> DSISLSLINEGPSYASKVSVGSNKQQQTVIIDTGSSDFWVVDSNAQCGKGVDCKSSGTFTPSSSSSYKNLGAAFTIRYGDGSTSQGTWGKDTVTINGVSITGQQIADVTQTSVDQGILGIGYTSNEAVYDTSGRQTTPNYDNVPVTLKKQGKIRTNAYSLYLNSPSAETGTIIFGGVDNAKYSGKLVAEQVTSSQALTISLASVNLKGSSFSFGDGALLDSGTTLTYFPSDFAAQLADKAGARLVQVARDQYLYFIDCNTDTSGTTVFNFGN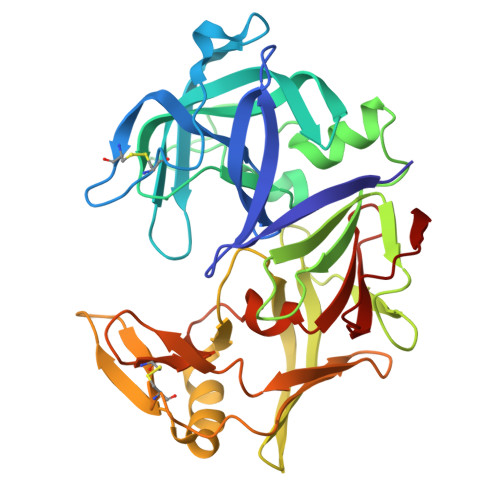GAKITVPNTEYVYQNGDGTCLWGIQPSDDTILGDNFLRHAYLLYNLDANTISIAQVKYTTDSSISAV>[2x]NFTQTLQKDANASSEFYINKLGQTQELEDQQTYKLLAARVLIRENKVEQSAALLRELGELNDAQKLDRALIEARISAAKNANEVAQNQLRALDLNKLSPSQKSRYYETLAIVAENRKDMIEAVKARIEMDKNLTDVQRHQDNIDKTWALLRSANTGVINNASDEGNAALGGWLTLIKAYNDYIRQPVQLSQALQSWKNAYPNHAAATLFPKELLTL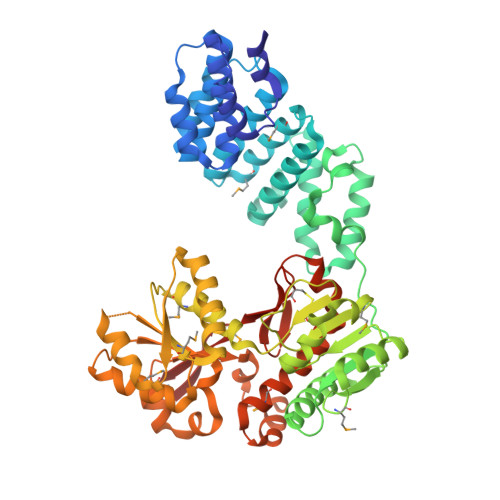LNFQQTNVSQIGLLLPLSGDGQILGTTIQSGFNDAKGNSTIPVQVFDTSMNSVQDIIAQAKQAGIKTLVGPLLKQNLDVILADPAQIQGMDVLALNATPNSRAIPQLCYYGLSPEDEAESAANKMWNDGVRNPLVAMPQNDLGQRVGNAFNVRWQQLAGTDANIRYYNLPADVTYFVQENNSNTTALYAVASPTELAEMKGYLTNIVPNLAIYASSRASASATNTNTDFIAQMNGVQFSDIPFFKDTNSPQYQKLAKSTGGEYQLMRLYAMGADAWLLINQFNELRQVPGYRLSGLTGILSADTNCNVERDMTWYQYQDGAIVPVAN Hazara virus (HAZV) is a member of the Bunyaviridae family of segmented negative stranded RNA viruses, and shares the same serogroup as Crimean-Congo haemorrhagic fever virus (CCHFV). The genomes of CCHFV and HAZV comprise three negative sense RNA segments, named small (S), medium (M) and large (L), which encode the nucleocapsid protein (N), the viral glycoproteins (Gn and Gc) and the viral RNA dependent RNA polymerase (L), respectively. As with all SNS RNA viruses, these RNA segments are encapsidated by the nucleocapsid protein (N) to form ribonucleoprotein (RNP) complexes. Genome encapsidation by N is required for multiple stages of the virus life cycle, including replication and transcription of the viral genome, as well as segment packaging during virus assembly.

We have determined the crystal structure of HAZV N to a resolution of 2.7 Å and found the structure of HAZV N to be very similar to the structure of CCHFV N, supporting the use of HAZV as a model for CCHFV infection. The crystallographic asymmetric unit (AU) contains four HAZV N monomers. In each of the four HAZV N monomers in the AU, only 475 amino acid residues were built into the model; residues 187–196 are missing in the electron density and are thought to form a disordered loop that links the arm domain to the N terminus of the globular domain. In agreement with the circular dichroism data, HAZV N is mostly alpha helical (helices are numbered according to Fig. 4b) and is composed of two distinct domains, a globular domain and an arm domain. Interestingly, HAZV N and the CCHFV N monomers in the AU of all three CCHFV N structures are packed in a similar way, with the base of the globular domain of one monomer making contact with residues on the arm domain of the adjacent monomer. HAZV N has a positively charged ‘platform’ adjacent to the arm domain (left) in a similar position to a positively charged platform on the surface of the CCHFV N protein. Superposition of HAZV N with CCHFV N strain Baghdad-12 reveals that the globular domains of these proteins align extremely closely (RMSD = 0.70 Å, over 368 residues that share 63 % sequence identity), as do the arm domains (RMSD = 0.89 Å over 107 residues that share 48 % sequence identity). The arm domain of CCHFV N is rotated by 74.0° around a pivot at serine 297 when compared with the arm domain of HAZV N resulting in a translation of 27.1 Å of the tip of the arm domain (the Cα of Asp 266).

>PLGSMENKIVASTKEEFNTWYKQFAEKHKLNNKYTESASFCAEIPQLDTYKYKMELASTDNERDAIYSSALIEATRFCAPIMECAWASCTGTVKRGLEWFDKNKDSDTVKVWDANYQKLRTETPPAEALLAYQKAALNWRKDVGFSIGEYTSILKKAVAAEYKVPGTVINNIKEMLSDMIRRRNRIINGGSDDAPKRGPVGREHLDWCREFASGKFLNAFNPPWGEINKAGKSGYPLLATGLAKLVELEGKDVMDKAKASIAQLEGWVKENKDQVDQDKAEDLLKGVRESYKTALALAKQSNAFRAQGAQIDTVFSSYYWLWKAGVTPVTFPSVSQFLFELGKNPKGQKKMQKALINTPLKWGKRLIELFADNDFTENRIYMHPCVLTSGRMSELGISFGAVPVTSPDDAAQGSGHTKAVLNYKTKTEVGNPCACIISSLFEIQKAGYDIESMDIVASEHLLHQSLVGKRSPFQNAYLIKGNATNINII[4x]> GAMGCVSSKSTTVLSPQTSFNEASRTSFRALPGPSQRQLEVYDQCLIGAARWPDDSSKSNTPENRAYCQSMYNSIRSAGDEIS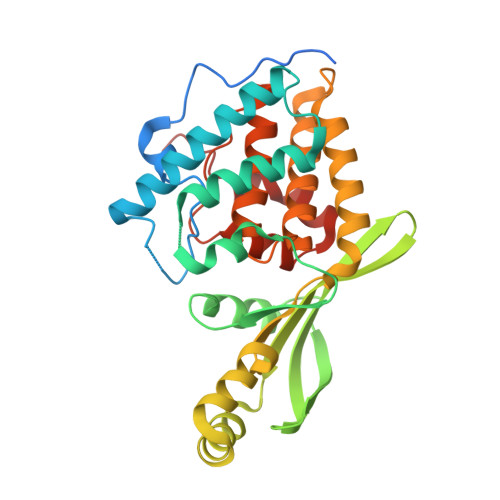RGGITSFEELWGRATEWRLSKLQRGEPLYSAFASERTSDTDAVTPLVKPYKSVLARVVDHEDAHDEIMQDNLFGDLNVKVYRQTAYLHGNVIPLNTFRVATDTEYLRDRVAHLRTELGAKALKQHLQRYNPDRIDHTNASYLPIIKDHLNDLYRQAISSDLSQAELISLIARTHWWAASAMPDQRGSAAKAEFAARAIASAHGIELPPFRNGNVSDIEAMLSGEEEFVEKYRSLLDSDCF(1~{S},2~{R})-2-[[(6-bromanyl-1~{H}-indazol-4-yl)amino]methyl]cyclohexan-1-ol | C14 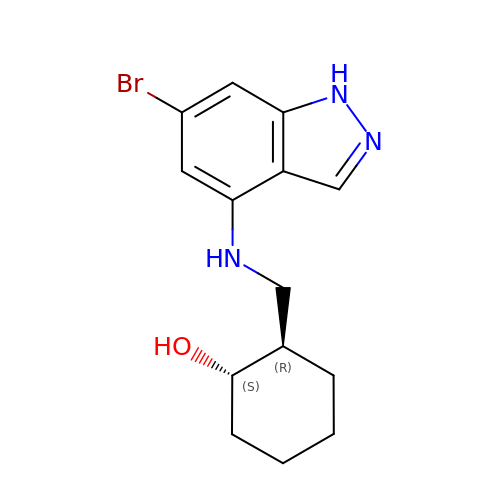H18 Br N3 O | KBSUKSFOQICUON-OTYXRUKQSA-N> AQIGPVTDLHITNANISPDGFSRPAVLAGGTFPGPT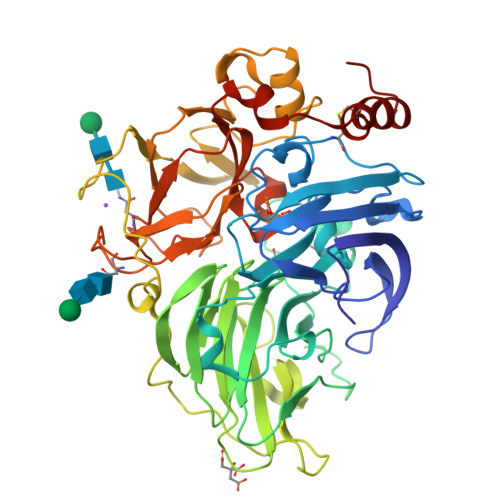IAGNTGDNFQITVFNDLTDPSMLTDTSIHWHGLFQKGTNWADGPAFVTQCPIITGQSFDYNFNVPGQAGTFWYHSHLSTQYCDGLRGPFVVYDPNDPNASLYDVDDDTTIITLADWYHTLAQQEPIGAAITADATLINGLGRSFTNTTASPLSVITVQSGKRYRMRLVSISCDPNYLFSIDGHDMTIIEVDGVNSQQLTVDQIQIFAAQRYSFVLNANQPVGNYWIRAQPNSGGQGFDGGINSAILRYEGATVEDPTTTAPTTFSNPLVETDLHPLADLGVPGQPFRGGADDPLVLNLAFANGRFSIDGVSFVPPTVPVLLQILSGAQNAQDLLPAGSVISLPSNSVIEVALPAGAAGGPHPFHLHGHNFAVVQSANNATPNYVNPIWRDTVSIGGTGDNVTIRFTTNNPGPWFLHCHIDWHLEAGFAIVFAEDIPDTASANPVPQAWSDLCPAYDQAHNIST> MKFDKPAGENPIDQLKVVGRPHDRIDGPLKTTGTARYAYEWHEEAPNAAYGYIVGSAIAKGRLTALDTDAAQKAPGVLAVITASNAGVLGKGDKNTARLLGGPTIEHYHQAIALVVAETFEQARAAASLVQAHYRRNKGAYSLADEKQAVNQPPEDTPDKNVGDFDGAFTSAAVKIDATYTTPDQSHMAMEPHASMAVWDGNKLTLWTSNQMIDWCRTDLAKTLKVPVENVRIISPYIGGGFGGKLFLRSDALLAALAARAVKRPVKVMLPRPSIPNNTTHRPATLQHLRIGADQSGKITAISHESWSGNLPGGTPETAVQQSELLYAGANRHTGLRLATLDLPEGNAMRAPGEAPGLMALEIAIDELAEKAGIDPVEFRILNDTQVDPAGPTRCFSRRQLIECLRTGADKFGWKQRNATPGQVRDGEWLVGHGVAAGFHNNLLEKSGARVHLEQNGTVTVETDMTDIGTGSYTILAQTAAEMLGVPLEQVAVHLGDSSFPVSAGSGGQWGANTSTSGVYAACMKLREMIASAVGFDPEQSQFADGKITNGTRSATLHEATAGGRLTAEESIEFGT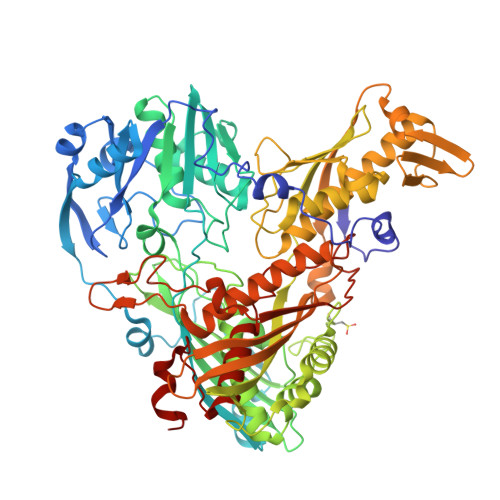LSKEYQQSTFAGHFVEVGVHSATGEVRVRRMLAVCAAGRILNPKTARSQVIGAMTMGMGAALMEELAVDDRLGYFVNHDMAGYEVPVHADIPKQEVIFLDDTDPISSPMKAKGVGELGLCGVSAAIANAVYNATGIRVRDYPITLDKLLDKLPDVV>[2x]MGVIVELIDHTSAIAAAKDRADLVERLRAAKARISDPQIRVVIAGQLKQGKSQLLNSLLNIPVARVGDDESTVLATVVSYGEQASARLVVARPDGAEPELIEIPPSEVTTDLRRAPQASGRQVLRVEVTAPSPLLKGGLAFVDTPGVGGHGQPHLSATLGLLPDADAMLMISDTSQEFTEPEMKFIRQALEICPVAAIVATKTDLYPHWRQIVDANIAHLQRAGLNVPV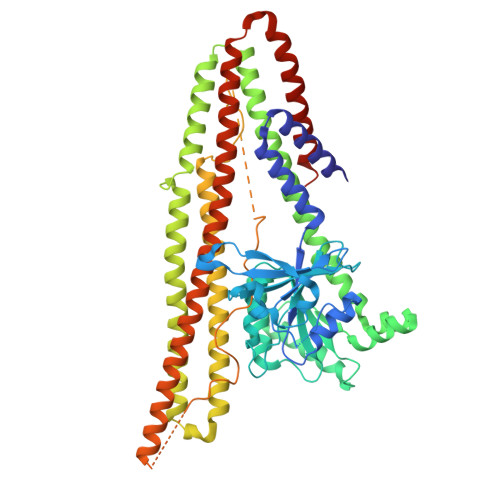IPASSVLRSHAISLNDKELNEESNFPAIVKFLSEHVLSRQNDRIRDQIVDEIRSAAEHLLLAVESELSSFNDPGERERLTAELERRKQEAQDALQQTALWQQVLSDGIADLTADVDHDLRHRFRIIAAHTEKVIDGCDPTLHWAEIGAELEDAVATAVGDNFVWAYQRAEALAAEVARTFTEAGLDAVQMPQIDARDMGAGFGELNSLARLEAKPIKIGHKVVTGMRGSYGGVLMFGMLTSFAGLGMFNPLSLGAGFVLGRKAYKEDMENRMLRVRNEAKANVRKFVDDVAFVVGKESRDRLKGIQRQLRDHYREIANQTTRSLNESLQAAIAAAKVEEAERNTRVKELERQQNILKQVVDHAAKLAAALEHHHHHH> MRQSHQLPLVGLLLFSFIPSQLCEICEVSEENYIRLKPLLNTMIQSNYNRGTSAVNVVLSLKLVGIQIQTLMQKMIQQIKYNVKSRLSDVSSGELALIILALGVCRNAEENLIYDYHLIDKLENKFQAEIENMEAHNGTPLTNYYQLSLDVLA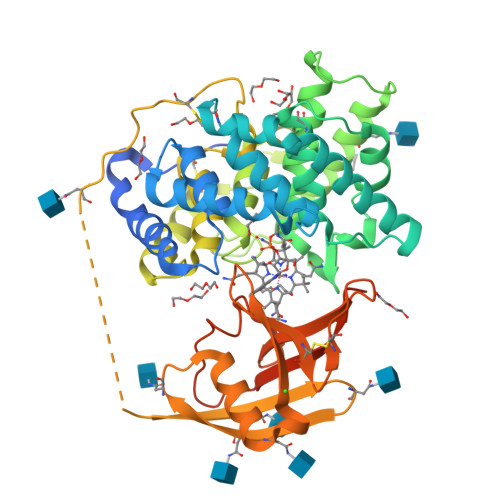LCLFNGNYSTAEVVNHFTPENKNYYFGSQFSVDTGAMAVLALTCVKKSLINGQIKADEGSLKNISIYTKSLVEKILSEKKENGLIGNTFSTGEAMQALFVSSDYYNENDWNCQQTLNTVLTEISQGAFSNPNAAAQVLPALMGKTFLDINKDSSCVSASGNFNISADEPITVTPPDSQSYISVNYSVRINETYFTNVTVLNGSVFLSVMEKAQKMNDTIFGFTMEERSWGPYITCIQGLCANNNDRTYWELLSGGEPLSQGAGSYVVRNGENLEVRWSKYLVPRGSLESRGPFEQKLISEEDLNMHTGHHHHHH>[2x]GPGDPHTYEDPNQAVLKFTTEIHPSCVTRQKVIGAGEFGEVYKGMLKTSSGKKEVPVAIKTLKAGYTEKQRVDFLGEAGIMGQFSHHNIIRLEGVISKYKPMMIITEYMENGALDKFLREKDGEFSVLQLVGMLRGIAAGMKYLANMNYVHRDLAARNILVNSNLVCKVSDFGLSRVLEDDPEATYTTSGGKIPIRWTAPEAISYRKFTSASDVWSFGIVMWEVMTYGERPYWELSNHEVMKAINDGFRLPTPMDCPSAIYQLMMQCWQQERARRPKFADIVSILDKLIRAPDSLKTLADFDPRVSIRLPSTSGSEGVPFRTVSEWLESIKMQQYTEHFMAAGYTAIEKVVQMTNDDIKRIGVRLPGHQKRIAYSLLGLKDQVNTVGIPI

The Eph receptors are the largest receptor tyrosine kinase family, and together with their cell surface-anchored ephrin ligands represent an important cell-cell communication system that regulates a multitude of physiological and pathological processes. The intracellular portion of the Eph receptors includes a juxtamembrane segment, the tyrosine kinase domain, a linker, a sterile alpha motif (SAM) domain, and a short C-terminal tail containing a PDZ domain-binding motif. EphA2 promotes cancer malignancy through a poorly understood non-canonical form of signaling involving serine/threonine phosphorylation of the linker connecting its kinase and SAM domains. The kinase-SAM linker contains a cluster of five serine/threonine residues that besides S897 include S892, T898, S899 and S901.

To obtain insights into EphA2 signaling mechanisms, we solved the crystal structure of most of the unphosphorylated EphA2 intracellular region (residues D590-I976). The crystallographic asymmetric unit contains two EphA2 molecules (molecules A and B), even though the EphA2 intracellular region is monomeric in solution. In our structure, the αA′-helix is unwound and Y594 (the second of two conserved juxtamembrane tyrosine residues) occupies a pocket previously found to be occupied by the first conserved tyrosine (Y588 in EphA2, which is not part of our construct), indicating a dynamic conformation of the juxtamembrane segment even when its tyrosine residues are unphosphorylated. The relative orientation of the kinase and SAM domains is different in the two EphA2 molecules, suggesting that the EphA2 intracellular region can assume different conformations, likely enabled by flexibility in the kinase-SAM linker. In contrast, residues S899-P905 (including the S899 and S901 phosphorylation sites) are mostly undefined in both EphA2 molecules, likely due to high conformational flexibility. Thus, conformational differences in these residues appear to be the main reason for the different relative orientations of the kinase and SAM domains in the two EphA2 molecules. In both EphA2 molecules, the N-terminal part of the linker is partly wrapped around the bottom of the kinase domain C-lobe and locked in place by interactions of I893 with a hydrophobic pocket in the kinase domain. This linker conformation is different from that observed in EphA2 structures that do not contain the SAM domain, where most of the linker (including I893) faces away from the kinase domain, suggesting that the SAM domain affects linker conformation. The correlation of the two exchange processes and the complementary charges of the two surfaces suggest that the kinase and SAM domains interact with each other, shielding the interacting surfaces from the solvent.>[2x]TILSDVKALGQQIWLDNLSRSLVQSGELAQMLKQGVSGVTSNPAIFQKAFAGDALYADEVAALKRQNLSPKQRYETMAVADVRAACDVCLAEHESTGGKTGFVSLEVSPELAKDAQGTVEEARRLHAAIARKNAMIKVPATDAGIDALETLVSDGISVNLTLLFSRAQTLKAYAAYARGIAKRLAAGQSVAHIQVVASFF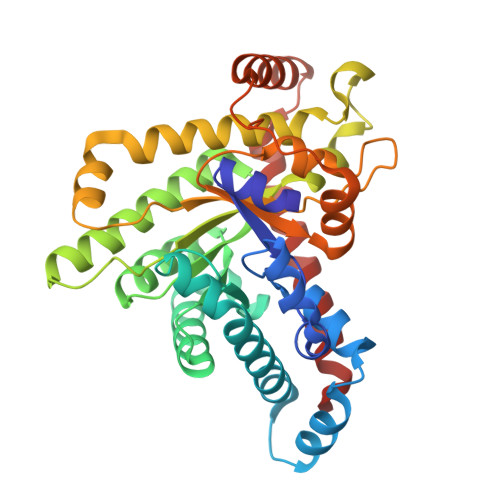ISRVDSALDATLPDRLKGKTAIALAKAAYQDWEQYFTAPEFAALEAQGANRVQLLWASTGVKNPAYPDTLYVDSLIGVHTVNTVPDATLKAFIDHGTAKATLTESADEARARLAEIAALGIDVETLAARLQEDGLKQFEEAFEKLLAPLV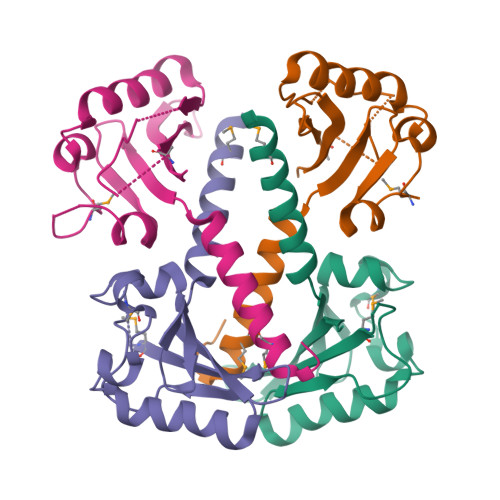>MHHHHHHENLYFQSNAMAKSRLLLSELLDQLSFALCIVRNDYVIVKVNEYFESRVIFDGETMQGKNILELFPESADYLKRKIDTALVIESSSFSSWEQKPHLLPFKSSRPVSGEEEQMYQNLEVIPIHSEDGTIEHVCLCVYDVTIQASQQQ[4x]> HP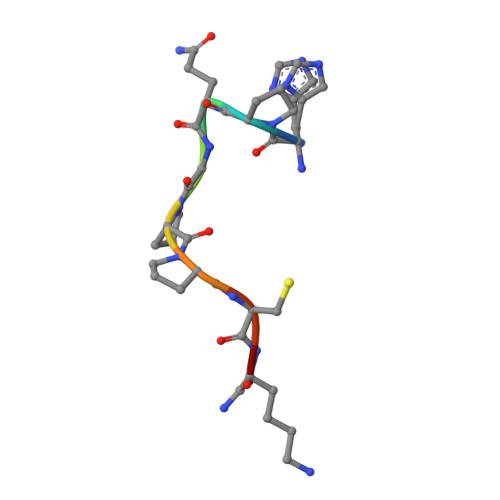QGPPCKX> MASSLGFGGSNAVDKVNATTTPGTVATPNSGPTKMLDEHILTPASISTLEVHGATNTRRSLLDQIFKPVLEDTAAAGTTLGQVLDRVGAATKKLARFDIFKE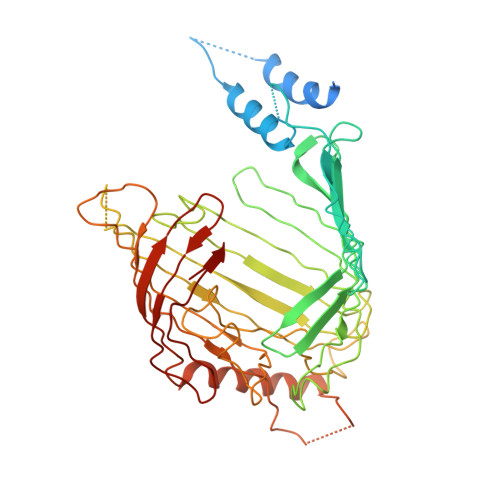EGFGVFLSEAAPPQSAPPTDRTDLDISIRVKEKSRLVFSAGTDFGNAEGSAYTNAVVRNIFGGAETLTVNASTGTRTRSAYNATFSTPINGNPDLRLSVEALRSATQKPWASHEEHLTGANLRLAWLTEKGDTHALAYSSVWRQLTGLAPTASPTVRADAGDSLKSSLTHTFTRDRRDNPMLPQSGYLFRSVSELAGWGPLNGDVSFAKTEVEASGALPVAIPGLAGKSGVSVGGGLRLGVLYPLPLGYSLTGAAQPSRINDRFQLGGPNDVRGFKIGGLGPHDGVDAVGGDVFAAGSVNALLPLPRTGPDSPLRLQLYANAGRLVALNSKGTDKEGKEGLAMDSAAVFKGVKSAVGKLTNGIPSLAAGVGLVYAHPVARFELNFSLPLVLRRGEEGRKGLQVGVGISFL>GETAPVSEPEGIGVALSIYPDGYGVNLYERPSDPIYAG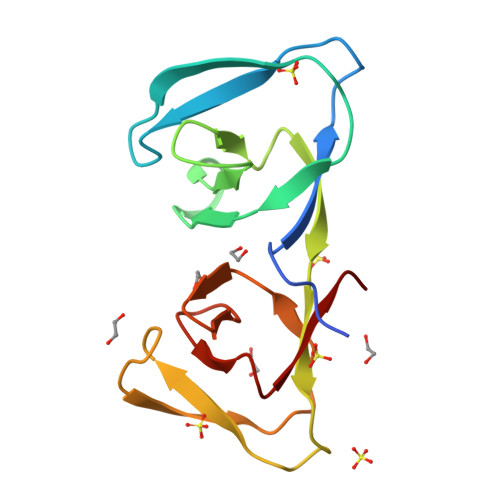NITKKIPYKVFAGYWGGGDKDMICLGGEKQWAYNKHFTIDWYKVRSKYPVGWGVNFYDGPSGNFLGNIDGSEVYNAHNRVGGYVDIGGNRWIKEEHVTITAK[2x]> MGRDPNSSSETSTETATVTLHKYVFDKSLPSDKIDNSKSQDEINAWLTKNNAEALDGVEFTAYDVTSEYADAYKTATGDKNESPADAAKTASAAVAKKADALQKTATVVGKQTTANGGLASFANLPLRDANGNYKAYLFAETDAPANITQKAEPFVLAMPIYGADGKTVQKSINIYPKNVKQSDKKTLNDNRSHHDFTAGEKINYSIETVVPWNIANKKVYTITDNPSKGLIMDADTIQIEGLASNKYTVKKNADNGFTITIPAANLAAFAGKTLKTTVKGHLSIEDLTLIDTGIPNKATAKVD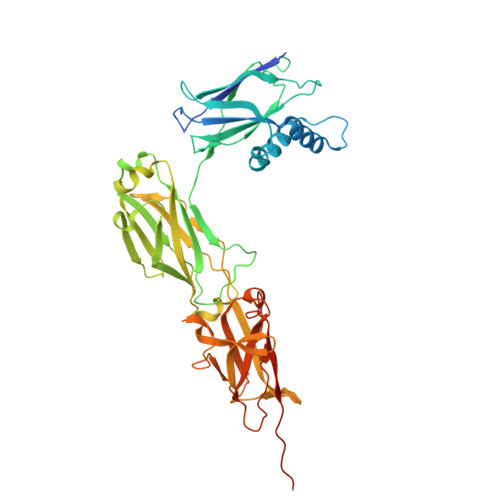NEAHHEVKSEEVFTGGKKFVKVDGSNQSKTLAGAQFQLVIVKNGQVVKYAHGNEKDGYTFDTNNTNVATKTTGENGQFEFAGLKYSESLEAGESYAVKEVKAPTGYDLLKDPVLFTVTKDSYKTVQAADGQKISNTKKGGFLPLEHHHHHH> MLSEVLLVSAPGKVILH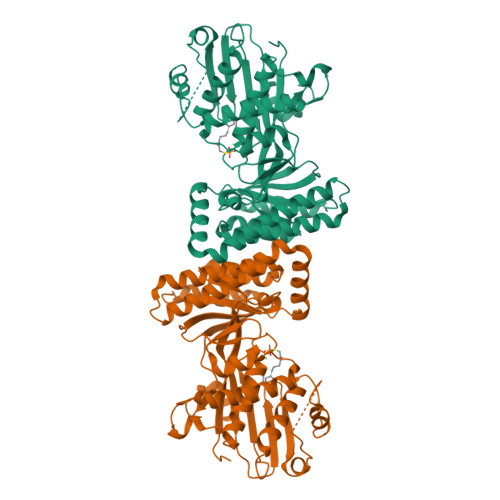GEHAVVHGKVALAVALNLRTFLVLRPQSNGKVSLNLPNVGIKQVWDVATLQLLDTGFLEQGDVPAPTLEQLEKLKKVAGLPRDCVGNEGLSLLAFLYLYLAICRKQRTLPSLDIMVWSELPPGAGLGSSAAYSVCVAAALLTACEEVTNPLKDRGSIGSWPEEDLKSINKWAYEGERVIHGNPSGVDNSVSTWGGALRYQQGKMSSLKRLPALQILLTNTKVPRSTKALVAGVRSRLIKFPEIMAPLLTSIDAISLECERVLGEMAAAPVPEQYLVLEELMDMNQHHLNALGVGHASLDQLCQVTAAHGLHSKLTGAGGGGCGITLLKPGLERAKVEAAKQALTGCGFDCWETSIGAPGVSMHSATSIEDPVRQALGL>[2x]MELCSGKPFDAFTDLKNGSLFAFRGQYSYELDEKAVRPGYPKLIRDVWGIEGPIDAAFTRINSQG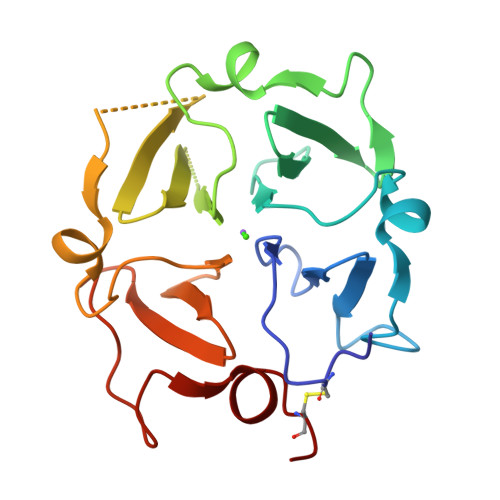KTYLFKGSQYWRFEDGVLDPDYPRNISDGFDGIPDNVDAALALPAHSYSGRERVYFFKGKQYWEYQFQRTSAGTRQPQFISRDWHGVPGQVDAAMAGRISVFFFSGDKYYRVNLRTRRVDTVDPPYPRSIAQYWLGCPA methyl 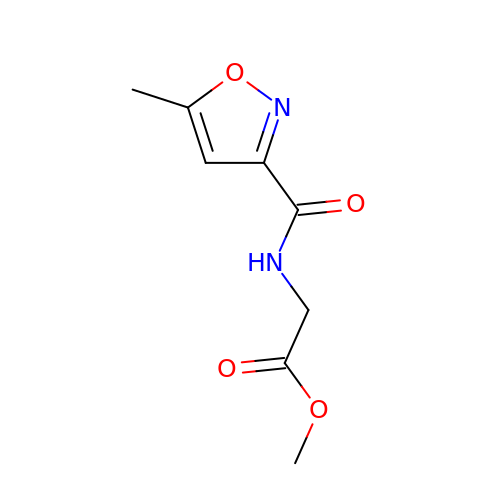N-(5-methyl-1,2-oxazole-3-carbonyl)glycinate | C8 H10 N2 O4 | FPAQMEYCJIMDCC-UHFFFAOYSA-N> MKRRVVITGVGVRAPGGNGTRQFWELLTSGRTATRRISFFDPSPYRSQVAAEADFDPVAEGFGPRELDRMDRASQFAVACAREAFAASGLDPDTLDPARVGVSLGSAVAAATSLEREYLLLSDSGRDWEVDAAWLSRHMFDYLVPSVMPAEVAWAVGAEGPVTMVSTGCTSGLDSVGNAVRAIEEGSADVMFAGAADTPITPIVVACFDAIRATTARNDDPEHASRPFDGTRDGFVLAEGAAMFVLEDYDSALARGARIHAEISGYATRCNAYHMTGLKADGREMAETIRVALDESRTDATDIDYINAHGSGTRQNDRHETAAYKRALG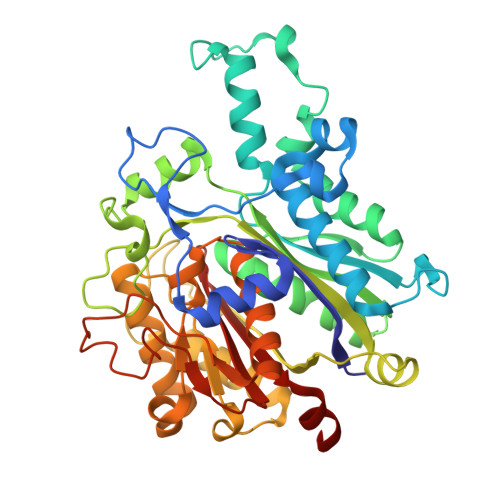EHARRTPVSSIKSMVGHSLGAIGSLEIAACVLALEHGVVPPTANLRTSDPECDLDYVPLEARERKLRSVLTVGSGFGGFQSAMVLRDAETAGAAA>SNAMSSVVVVGTQWGDEGKGKITDFLSEHAEVVARYQGGNNAGHTIVFGGVKYKLHLIPSGIFYKEKICVIGNGLVVDPKALLEELKYLHDRGVSTDNLRVSNRAHVILPYHLKQDELEEASKGDNKIGTTKKGIGPAYMDKAARIGIRMADLLDREAFKEKLEQNLAQKNRLFEKMYDTEGFSVDEIFEEYFEYGQQIAQYVCDTSVVLNDALDNNHRVLFEGAQGVMLDIDHGTYPFVTSSNPIAGGVTVGTGVGPAKVTRVVGVCKAYTSRVGDGPFPTELHDEIGHQIREVGREYGTTTGRPRRVGWFDSVVVRHARRVSGLTDLSLNSIDVLTGIPTLKICVAYKCDGKVIDEVPANLNILAKCEPVCEEL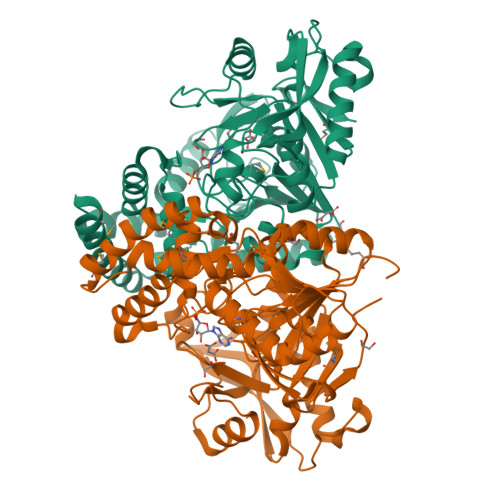PGWTEDITGVRSLDELPENARKYVERVSELTGIQLSMFSVGPDRNQTNIVRNVYEA[2x]> PQVWQLISKVLARHFSAADASRVLEQLQRDYE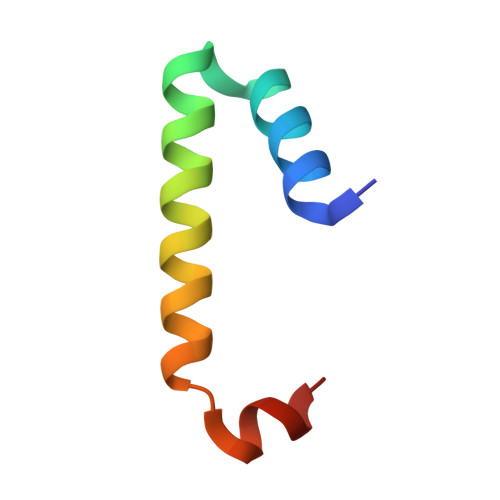RSLSRLTLDDIERLA> MRVLVTGGSGYIGSHTCVQLLQNGHDVIILDNLCNSKRSVLPVIERLGGKHPTFVEGDIRNEALMTEILHDHAIDTVIHFAGLKAVGESVQKPLEYY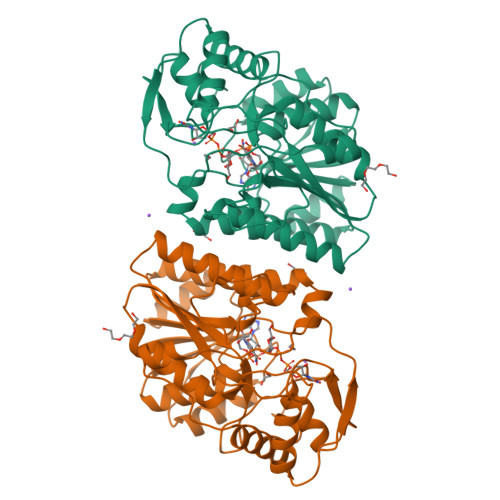DNNVNGTLRLISAMRAANVKNFIFSSSATVYGDQPKIPYVESFPTGTPQSPYGKSKLMVEQILTDLQKAQPDWSIALLRYFNPVGAHPSGDMGEDPQGIPNNLMPYIAQVAVGRRDSLAIFGNDYPTEDGTGVRDYIHVMDLADGHVVAMEKLANKPGVHIYNLGAGVGNSVLDVVNAFSKACGKPVNYHFAPRREGDLPAYWADASKADRELNWRVTRTLDEMAQDTWHWQSRHPQGYPD> MPYIEKLELKGFKSY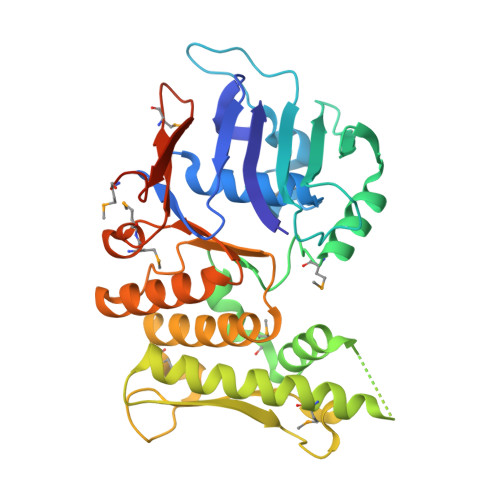GNKKVVIPFSKGFTAIVGANGSGKSNIGDAILFVLGGLSAKAMRASRISDLIFAGSKNEPPAKYAEVAIYFNNEDRGFPIDEDEVVIRRRVYPDGRSSYWLNGRRATRSEILDILTAAMISPDGYNIVLQGDITKFIKMSPLERRLLIDDISGIAEYDSKKEKALEEEKEKKNVFMRTFEAISRNFSEIFAKLSPGGSARLILENPEDPFSGGLEIEAKPAGKDVKRIEAMSGGEKALTALAFVFAIQKFKPAPFYLFDEIDAHLDDANVKRVADLIKESSKESQFIVITLRDVMMANADKIIGVSMRDGVSKVVSLSLEKAMKILEEIRKKQGWEHGN>MLSKTILDKLNHQVNFEAASAHLYLQMSAWLLTQSLDSTAAFFRAHAEEEKAHMMKLFDYINETGSLALIGEVATPAPEWKSHIELLEAAYNHELAITQSINDLVDTALREKDYSTFQFLQWYVAEQHEEEYLFSSMLHKARIINTMDGRALFRFDEEVRKSVLHHEHHQQKPMFLQVGPAPKHHDGHDGLHAHQHSSHWSGH[23x];> MLSKTILDKLNHQVNFEAASAHLYLQMSAWLLTQSLDSTAAFFRAHAEEEKAHMMKLFDYINETGSLALIGEVATPAPEW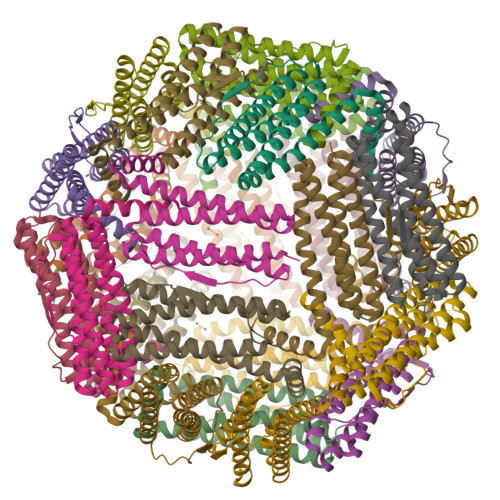KSHIELLEAAYNHELAITQSINDLVDTALREKDYSTFQFLQWYVAEQHEEEYLFSSMLHKARIIDTMDGRALFRFDEEVRKSVLHHEHHQQKPMFLQVGPAPKHHDGHDGLHAHQHSSHWSGH>[2x]MYSKIKISGTIEVVTGLHIGG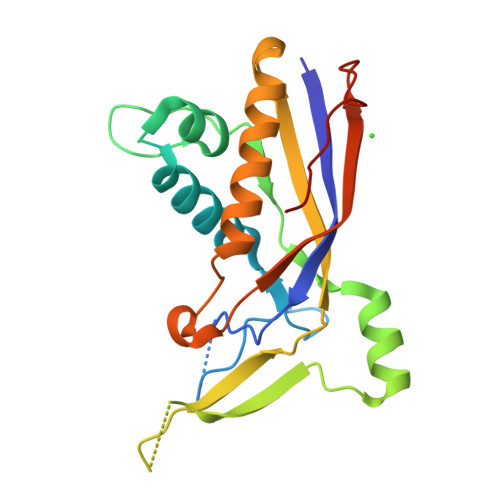GGESSMIGAIDSPVVRDLQTKLPIIPGSSIKGKMRNLLAKHFGLKMKQESHNQDDERVLRLFGSSEKGNIQRARLQISDAFFSEKTKEHFAQNDIAYTETKFENTINRLTAVANPRQIERVTRGSEFDFVFIYNVDEESQVEDDFENIEKAIHLLENDYLGGGGTRGNGRIQFKDTNIETVVGEYDSTNLKIKAALEHHHHHH> MGHHHHHHHHHHMQSSVNEFLTPRHIDVQVVSQTRAKITLEPLERGFGHTLGNALRRILLSSMPGCAVVEAEIDGVLHEYSAIEGVQEDVIEILLNLKGLAIKLHGRDEVTLTLAKKGSGVVTAADIQLDHDVEIINGDHVIANLADNGALNMKLKVARG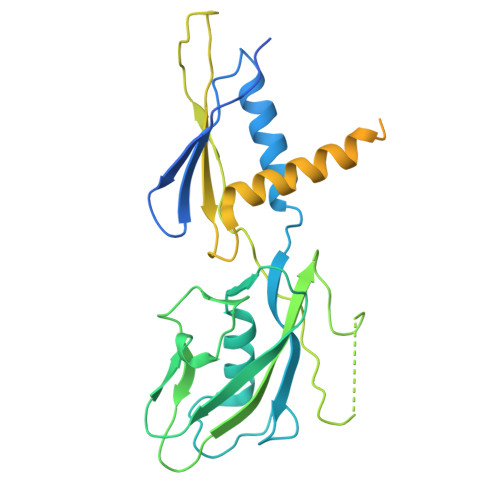RGYEPADARQSDEDESRSIGRLQLDASFSPVRRVSYVVENARVEQRTNLDKLVLDLETNGTLDPEEAIRRAATILQQQLAAFVDLKGDSEPVVEEQEDEIDPILLRPVDDLELTVRSANCLKAENIYYIGDLIQRTEVELLKTPNLGKKSLTEIKDVLASRGLSLGMRLDNWPPASLKKDDKATA>PRERPHTSGHHGAGEARATAPSTVSPYGPEARAELSSRLTTLRNTLAPATN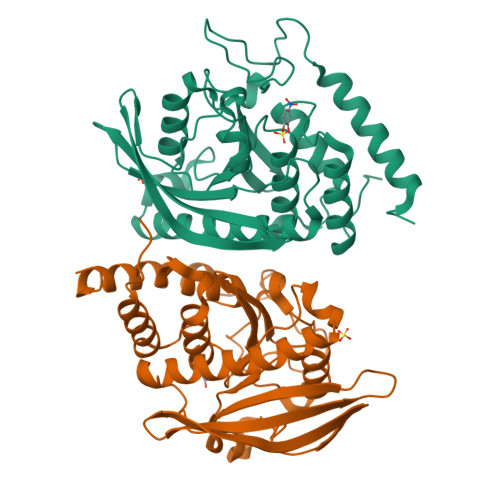DPRYLQACGGEKLNRFRDIQCRRQTAVRADLNANYIQVGNTRTIACQYPLQSQLESHFRMLAENRTPVLAVLASSSEIANQRFGMPDYFRQSGTYGSITVESKMTQQVGLGDGIMADMYTLTIREAGQKTISVPVVHVGNWPDFTAVSSEVTKALASLVDQTAETKRNMYESKGSSAVADDSKLRPVIHCRAGVGRTAQLIGAMCMNDSRNSQLSVEDMVSQMRVQRNGIMVQKDEQLDVLIKLAEGQGRPLLNS[2x]>[2x]MASVAQPVRRR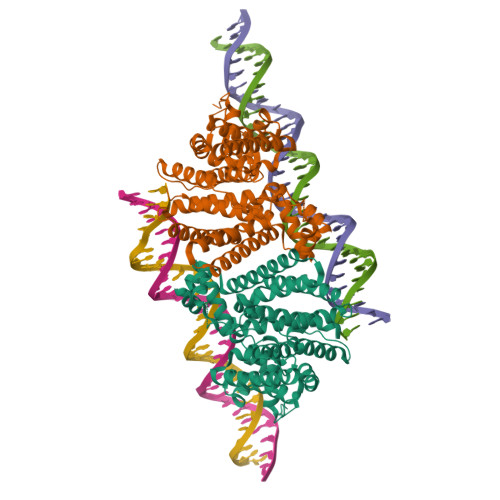PKDRKKQILDQAVGLFIERGFHSVKLEDIAEAAGVTARALYRHYDNKQALLAEAIRTGQDQYQSARRLTEGETEPTPRPLNADLEDLIAAAVASRALTVLWQREARYLNEDDRTAVRRRINAIVAGMRDSVLLEVPDLSPQHSELRAWAVSSTLTSLGRHSLSLPGEELKKLLYQACMAAARTPPVCELPPLPAGDAARDEADVLFSRYETLLAAGARLFRAQGYPAVNTSEIGKGAGIAGPGLYRSFSSKQAILDALIRRLDEWRCLECIRALRANQQAAQRLRGLVQGHVRISLDAPDLVAVSVTELSHASVEVRDGYLRNQGDREAVWIDLIGKLVPATSVAQGRLLVAAAISFIEDVARTWHLTRYAGVADEISGLALAILTSGAGNLLRA> MRGSHHHHHHGMASMNEFPVVLVINCGSSSIKFSVLDVATCDVLMAGIADGMNTENAFLSINGDKPINLAHSNYEDALKAIAFELEKRDLTDSVALIGHRIVHGGELFTQSVIITDEII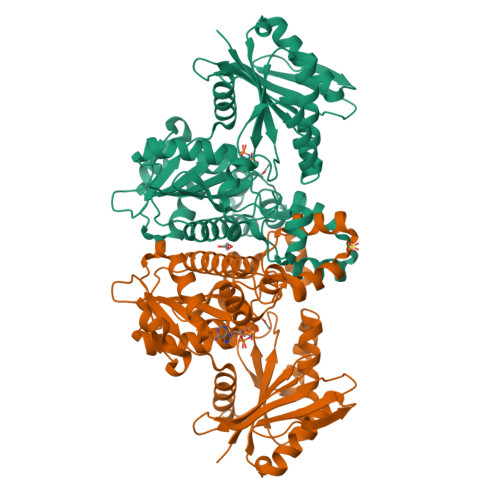DNIRRVSPLAPLHNYANLSGIDAARHLFPAVRQVAVFDTSFHQTLAPEAYLYGLPWEYFSSLGVRRYGFHGTSHRYVSRRAYELLDLDEKDSGLIVAHLGNGASICAVRNGQSVDTSMGMTPLEGLMMGTRSGDVDFGAMAWIAKETGQTLSDLERVVNKESGLLGISGLSSDLRVLEKAWHEGHERARLAIKTFVHRIARHIAGHAASLHRLDGIIFTGGIGENSVLIRQLVIEHLGVLGLTLDVEMNKQPNSHGERIISANPSQVICAVIPTNEEKMIALDAIHLGNVKAPVEFA>MIVRNLGDIRKTDRNVRSDGWASARMLLKDDGMGFSFHVTTLFAGSELRMHYQNHLEAVLVLKGTGTIEDLATGEVHALRPGVMYALDDHDRHIVRPETDILTACVFNPPVTGREVHDESGAYPADP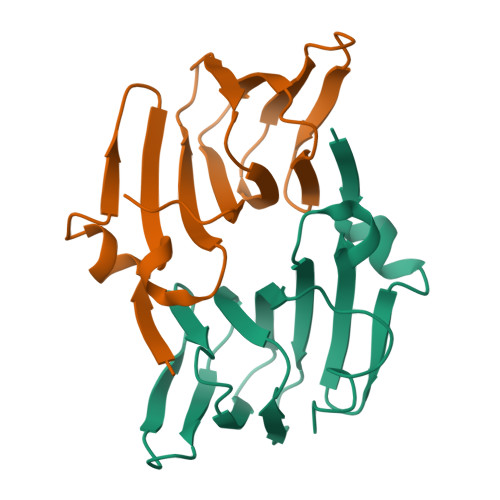ELAREPVAADNWSHPQFEK[4x]1H-INDOLE-3-CARBALDEHYDE | C9 H7 N O | 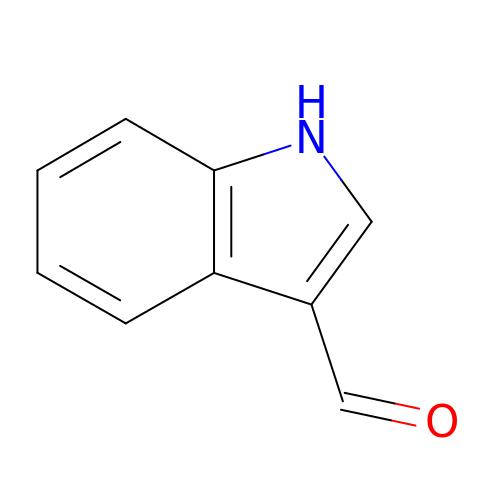OLNJUISKUQQNIM-UHFFFAOYSA-N> MLTEGISIQSYDGHTFGALVGSPAKAPAPVIVIAQEIFGVNAFMRETVSWLVDQGYAAVCPDLYARQAPGTALDPQDEAQREQAYKLWQAFDMEAGVGDLEAAIRYARHQPYSNGKVGLVGYSLGGALAFLVAAKGYVDRAVGYYGVG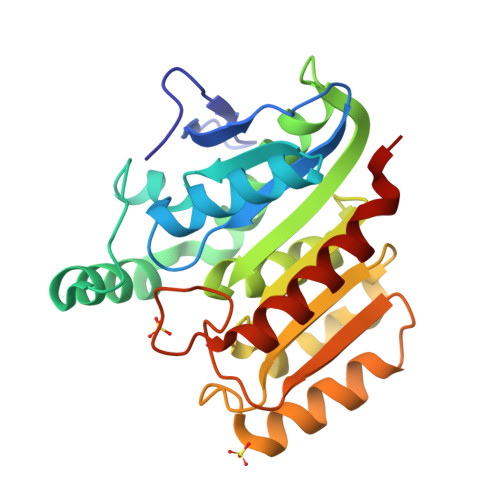LEKQLNKVPEVKHPALFHMGGQDHFVPAPSRQLITEGFGANPLLQVHWYEEAGHSFARTSSSGYVASAAALANERTLDFLAPLQSKKP>[6x]GSHMATEKVTKDVASDLAGQVKFVNLDAEEKRDRQGTTTRIAPKGGLIWVLSGEVYNLPPGAEPVVKNGDRIEAGAVMAETTVKTEHGGVVRLPEQQDSKGGREVEIITASVMLDKAKVLKETQQGREHYIIETATGQRFSLKAAPGTKVANGQVVAELIDDRYHTTTGGILKYADIEVAKKGKAKQGYEVLKGGTLLWIPEETHEVNKDISLLMVEDNQYVEAGTEVVKDIFCQNSGVVEVIQKNDILREIIIKPGELHLVDDPEAARLKHGTLARPGEEVLPGLVVDTLSQVDYLEDTPEGPAILMRPVQEFSVPDEPSVPSQDSSDGSGQSIRLRAVQRLPYKHDERVKSVDGVDLLRTQLVLEIGSEAP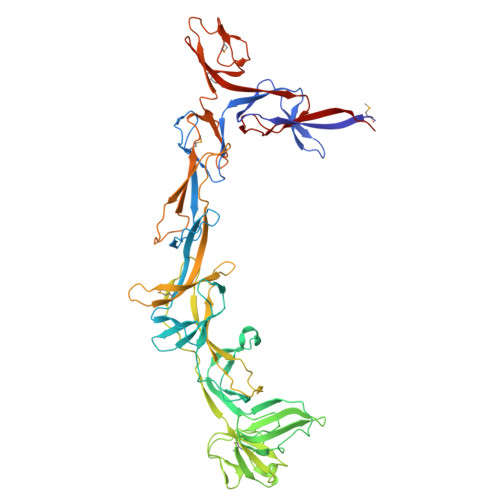QLAADIEIVTDEVDPEAQRLQLVILESLIIRRDIAADQTQGSTFTSLLVKDGDHIGPGAVIARTDIKAKQAGEVQGIVRSGESVRRILVVTDSDRLRVETNGAKPTVKVGDLVRPGDEMAKGVTAPETAAVMAVADDHVILRLARPYLVSPGAVLQIEEGDLVQRGDNLALLVFERAKTG> VVVTGYTTQRKADLTGAVSVVKVDEIQKQGENNPVKALQGRVPGMNITADGNPSGSATVRIRGIGTLNNNDPLYIIDGVPTKAGMHELNGNDIESIQVLKDAASASIYGSRAANGVIIITTKQGKKGQIKINFDASVSASMYQSKMNVLNTEQYGRAMWQAYVNDGE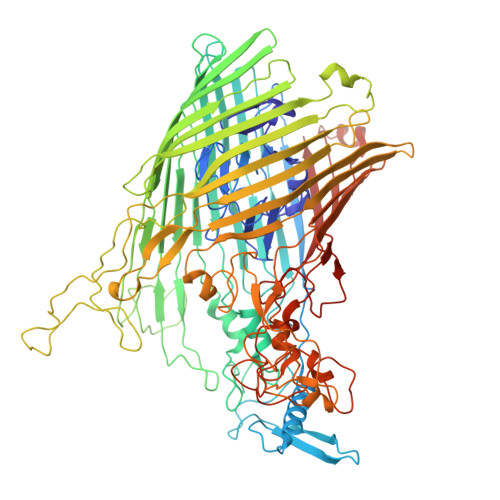NPNGNALGYAYNWGYNADGNPVLYGMTLSKYLDSKNTMPVADTDWFDEITRTGVIQQYNLSVSNGSEKGSSFFSLGYYKNLGVIKDTDFDRFSARMNSDYKLIDDILTIGQHFTLNRTSEVQAPGGIIETALDIPSAIPVYASDGSWGGPVGGWPDRRNPRAVLEYNKDNRYTYWRMFGDAYVNLTPFKGFNLRSTFGLDYANKQARYFTYPYQEGTQTNNGKSAVEAKQEHWTKWMWNAIATYQLEVGKHRGDVMIGMELNREDDSHFSGYKEDFSILTPDYMWPDAGSGTAQAYGAGEGYSLVSFFGKMNYSYADRYLLSLTLRRDGSSRFGKNHRYATFPSVSLGWRITQENFMKELTWLDDLKLRASWGQTGNQEISNLARYTIYAPNYGTTDSFGGQSYGTAYDITGSNGGGVLPSGFKRNQIGNDNIKWETTTQTNVGIDFSLFKQSLYGSLEYYYKKATDILTEMAGVGVLGEGGSRWINSGAMKNQGFEFNLGYRNKTAFGLTYDLNGNISTYRNEILELPETVAANGKFGGNGVKSVVGHTYGAQVGYIADGIFKSQDEVDNHATQEGAAVGRIRYRDIDHNGVIDERDQNWIYDPTPSFSYGLNIYLEYKNFDLTMFWQGVQGVDIISDVKKKSDFWSASNVGFLNKGTRLLNAWSPTNPNSDIPALTRSDTNNEQRVSTYFVENGSFLKLRNIQLGYTVPAVISKKMRMDRLRFYCSAQNLLTIKSKNFTGEDPENPNFSYPIPVNITFGLNIGF>[4x]MRVLVSNDDGVDAPGIKILADALRNAGHEVMVVAPDRDRSGASNSLTLDTPIRAKQIDMHTYSVAGTPTDCVHLALTG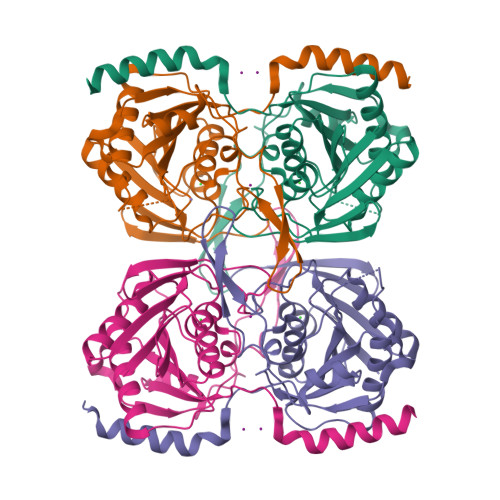LLNYDPDIVVSGINNTGNLGDDVIYSGTVSAAMEGRFLGLPAVAVSLVTLYREGQQAPQYETAAHAAINIVAQLKTDPLPADTILNVNVPDVTWQQMRGFKVTRLGNRHRSAPCLTQTDPRGHTIYWIGPAGPEQDAGPGTDFDAVRNTYISITPIHVDLTRYQALENVTRWTDRLTAHMDWPTLEHHHHHH> PGPPQGPPQPVQQSKRLQQTQAQVEEVVDIMRVNVDKVLERDSKISELDDRADALQAGASQFEASAGKLKRKFWWKNCKM;> GKSASGIIMETQQAKQTLADIEARHADIMKLETSIRELHDMFMDMAMLVESQGEMIDRIEYNVEAAVDYIETAKVDTKKAVKYQSKAR;> NGEVEVPKTELEEIQQQCNQVTDDSLESTRRMLNMCEESKEAGIRTLVMLDEQGEQLDRIEEGLDQINQDMKDAEKNLEGMEK;> VTVGDQNGMGPSSGYVTRITNDAREDDMENNMKEVSSMIGNLRNMAIDMGNEIGSQNRQVDRIQQKAESNESRIDEANKKATKLLKN;> GKSASGEKEGNENAEEEAAAIEEARRE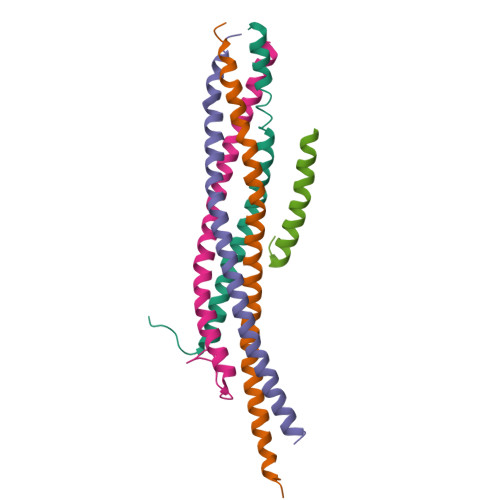AEERRKEKHRKMEEEREEMRQTIRDKYGLKKKVKEEPEAEADLDEGRVGRKK>[2x]APITAYSQQTRGLLGCIITSLTGRDKNQVDGEVQVLSTATQSFLATCVNGVCWTVYHGAGSKTLAGPKGPITQMYTNVDQDLVGWPAPPGARSMTPCTCG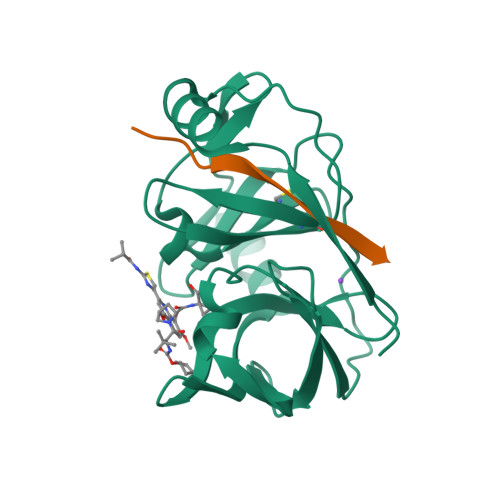SSDLYLVTRHADVIPVRRRGDSRGSLLSPRPVSYLKGSSGGPLLCPSGHVVGIFRAAVCTRGVAKAVDFIPVESMETTMRASKKKK;>KKGSVVIVGRIILSGRK[2x]>ETGKHNCFCIQEVVSGLRQPVGALHSGDGSQRLFILEKEGYVKILTPEGEIFKEPYLDIHKLVQSGIKGGDERGLLSLAFHPNYKKNGKLYVSYTTNQERWAIGPHDHILRVVEYTVSRKNPHQVDLRTARVFLEVAELHRKHLGGQLLFGPDGFLYIILGDGMITLDDMEEMDGLSDFTGSVLRLDVDTDMCNVPYSIPRSNPHFNSTNQPPEVFAHGLHDPGRCAVDRHPTDININLTILCSDSNGKNRSSARILQIIKGKDYESEPSLLEFKPFSNGPLVGGFVYRGCQSERLYGSYVFGDRNGNFLTLQQSPVTKQWQEKPLCLGTSGSCRGYFSGHILGFGEDELGEVYILSSSKSMTQTHNGKLYKIVDPKRPLMPEECRATVQPAQTLTSECSRLCRNGYCTPTGKCCCSPGWEGDFCRTAKCEPACRHGGVCVRPNKCLCKKGYLGPQCEQVDGTK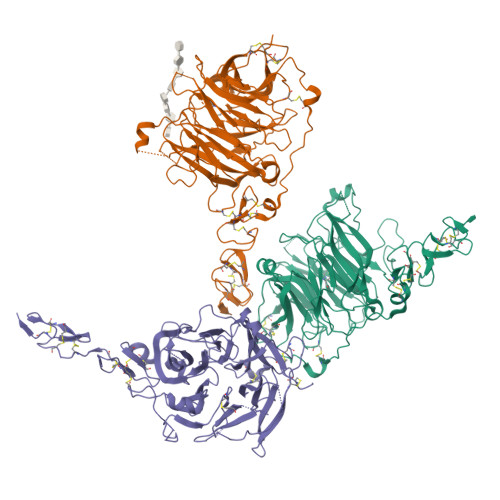HHHHHH[3x]> SMAL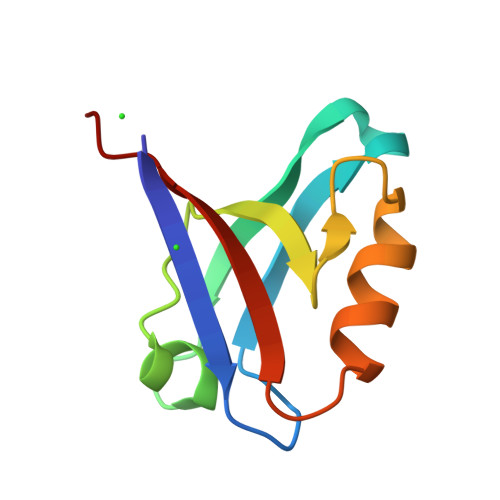TVDVAGPAPWGFRITGGRDFHTPIMVTKVAERGKAKDADLRPGDIIVAINGESAEGMLHAEAQSKIRQSPSPLRLQLDRITSL> GAMSNIYIQEPPTNGKVLLKTTAGDIDIELWSKEAPKACRNFIQLCLEAYYDNTIFHRVVPGFIVQGGDPTGTGSGGESIYGAPFKDEFHSRLRFNRRGLVAMANAGSHDNGSQFFFTLGRADELNNKHTIFGKVTGDTVYNMLRLSEVDIDDDERPHNPHKIKSCEVLFNPFDDIIP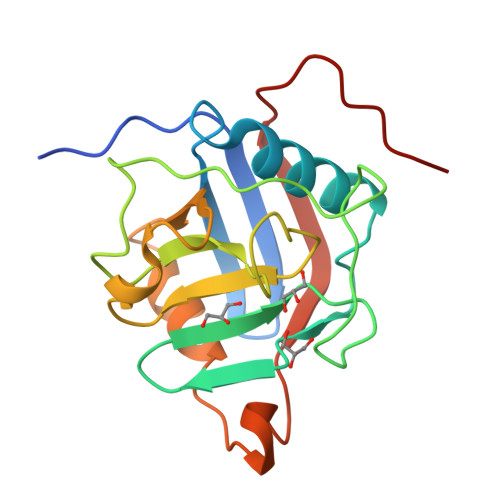RE>[2x]ADKLPNIVILATGGTIAGSAATGTQTTGYKAGALGVDTLINAVPEVKKLANVKGEQFSNMASENMTGDVVLKL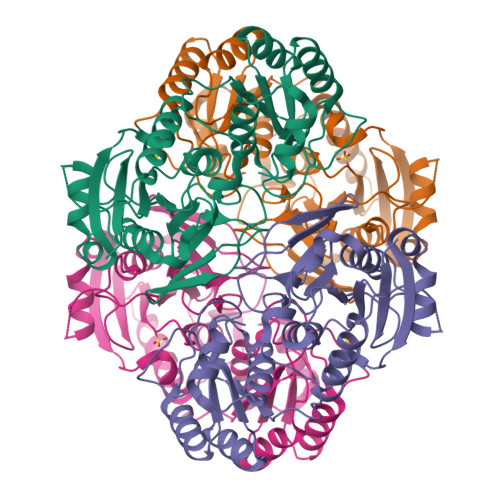SQRVNELLARDDVDGVVITHGTDTVEESAYFLHLTVKSDKPVVFVAAMRPATAISADGPMNLLEAVRVAGDKQSRGRGVMVVINDRIGSARYITKTNASTLDTFRANEEGYLGVIIGNRIYYQNRIDKLHTTRSVFDVRGLTSLPKVDILYGYQDDPEYLYDAAIQHGVKGIVYAGMGAGSVSVRGIAGMRKALEKGVVVMRSTRTGNGIVPPDEELPGLVSDSLNPAHARILLMLALTRTSDPKVIQEYFHTY>MIHMRTGVIGVGHLGRFHAQKYAAISQLAGVFDENAERAAEVAAELRCRAFPSVDALLAEVDAVSIVTPTSTHFAVAEVAMQAGVHCLIEKPFTLDTEEADALIGMAQERHLVLAIGHIKRVHPAIQYLRQAGFGAPRYLEAERLAPFKPRSLDIDVIMDLMIHDLDLTLLLTGAEPVDVRAVGVAAVTDKADMATAWMTLNNGTVANLAASRVVREPARRMRIFWQDRYASVDFLNNTLHIYHRGAGTVPGIPGVRDEAVDLAKRDALAAEIEDFLNAIAAHRPVFCDG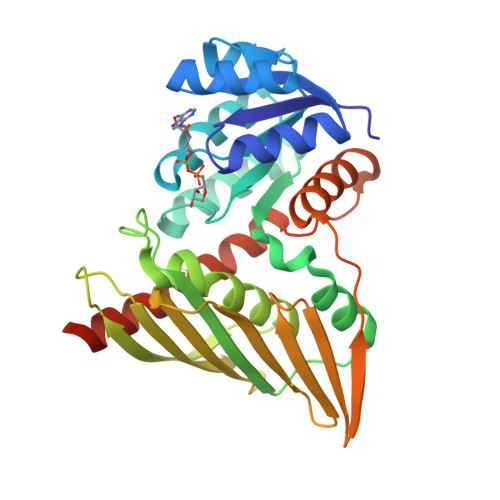VAGRRVLAAALQVRVAVEAFLQRLEHHHHHH[2x]>CGCG[2x];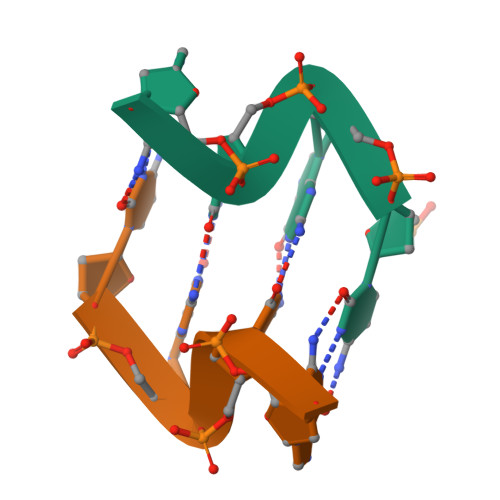>GCGC[2x]>[4x]MTEHPRAHTAHLRTARLELTPLDPAADARHLHHAYGDEEVMRWWTRPACADPAETERYLT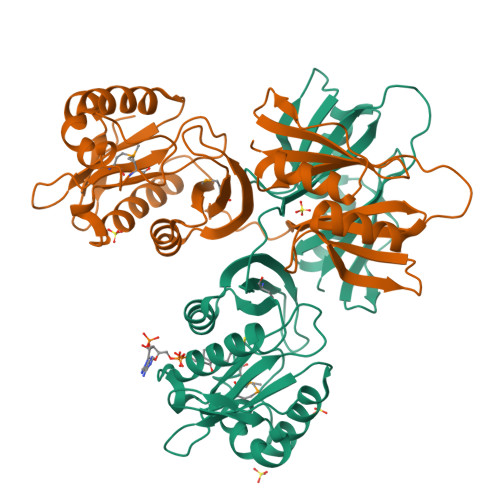SCAAAPGARLWTIRAPDGTVPGMAGLLGGTDVPGLTWLLRRDSWGHGYATEAAAAVVGHALEDGGLDRVEAWIEAGNRRSLAVAARVGLTERARLAQHYPHRPGPHEMVVLGKARAEEPLTTLAVITELPVRDVAATLRLVEAALGARTAFAIGDPPEFAEAALTPWSAGPRFRLAAVPGPGPVEPVRLHLDAAGTADSLHRRAVDAGARVDGPPVRRPWGRSEFVITLPEGHELTVSAPV>[20x]MNELEGYVT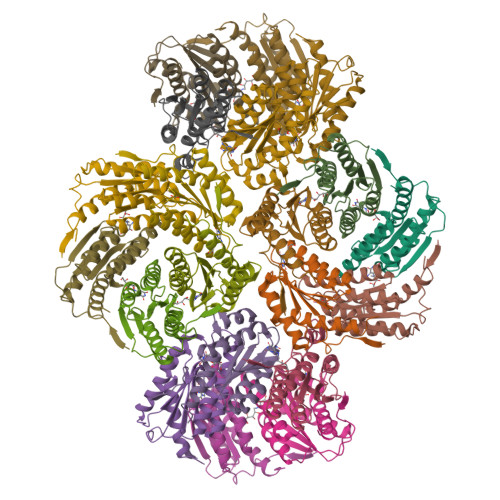KAQSFRFAIVVARFNEFVTRRLMEGALDTFKKYSVNEDIDVVWVPGAYELGVTAQALGKSGKYHAIVCLGAVVKGDTSHYDAVVNSASSGVLSAGLNSGVPCVFGVLTCDNMDQAINRAGGKAGNKGAESALTAIEMASLFEHHLKA> MAFARGGLAQTASQTTSSPVRVGLSVDASALGHTIPPDYTGLSYEQAQMANPNYFSGANTQLAGFLRTLGRQGVLRIGGNTSEYTFWNRHAKPTAADEHLAAGPDKGHHAAAREVITPEAVNNLSEFLDKTGWKLIYGLNLGKGTPENAADEAAYVMETIGADRLLAFQLGNEPDLFYRNGIRPASYDFAAYAGDWQRFFTAIRKRVPNAPFAGPDTAYNTKWLVPFADKFKHDVKFISSHYYAEGPPTDPSMTIERLMKPNPRLLGETAGLKQVEADTGLPFRLTETNSCYQGGKQGVSDTFAAALWAGDLMYQQAAAGSTGINFHGGGYGWYTPVAGTPEDGFIARPEYYGMLLFAQAGAGQLLGAKLTDNSAAPLLTAYALRGTDGRTRIALFNKNLDADVEVAISGVASPSGTVLRLEAPRADDTTDVTFGGAPVGASGSWSPLVQEYVPGHSGQFVLHMRKASGALLEFA

Siastatin B is a potent and effective iminosugar inhibitor of three diverse glycosidase classes, namely, sialidases, β-d-glucuronidases, and N-acetyl-glucosaminidases. Surprisingly, siastatin B also inhibits both β-glucuronidases and human heparanase, which cleave β-glucuronic acid residues but not sialic acid or N-acetylated sugars. Herein, we show through crystallographic analysis of protein-inhibitor complexes that siastatin B generates both a hemiaminal and a 3-geminal diol iminosugar (3-GDI) that are, rather than the parent compound, directly responsible for enzyme inhibition. Notably, 3-GDIs are a new class of iminosugar glycoside hydrolase inhibitor, that have been shown to inhibit both GH2 and GH79 β-glucuronidases.

However, we were surprised to find that although each of the structures contains a ligand present with full occupancy in the active site, none of the observed ligands are siastatin B. Three of the four enzymes (AcGH79, BpHEP, and EcGusB) contained “galacturonic-noeuromycin” bound in the −1 position of the active site, as opposed to siastatin B. We confirmed the presence of an alcohol at the 2-position–as opposed to an amine, which would result from deacetylation–through examination of the B-factors within the high-resolution crystal structures of AcGH79 and BpHEP, see Figure S4. When the 2-position is modeled as an alcohol, the B-factor of the 2-substituent is consistent with the 2-carbon. However, when the 2-position is modeled as an amine, the B-factor of this functional group is depressed, which is anticipated for a nitrogen being accommodated within the electron density of an oxygen. The 2-hydroxyl is within hydrogen bonding distance of the catalytic nucleophile and an active site asparagine in all three of these structures, thereby mimicking the interactions seen for natural substrates28 and other inhibitors. The 4-hydroxyl of 4 has galacto-stereochemistry in contrast to the gluco-configuration of the natural enzyme substrate; however, this position also appears to have productive binding to the active site. The 4-hydroxyl of 4 forms hydrogen bond interactions with the enzyme active site, for both AcGH79 and EcGusB, see Figure 2AC.> MYNMRRLSLSPTFSMGFHLLVTVSLLFSHVDHVIAETEMEGEGNETGECTGSYYCKKGVILPIWEPQDPSFGDKIARATVYFVAMVYMFLGVSIIADRFMSSIEVITSQEKEITIKKPNGETTKTTVRIWNETVSNLTLMALGSSAPEILLSVIEVCGHNFTAGDLGPSTIVGSAAFNMFIIIALCVYVVPDGETRKIKHLRVFFVTAAWSIFAYTWLYIILSVISPGVVEVWEGLLTFFFFPICVVFAWVADRRLLFYKYVYKRYRAGKQRGMIIEHEGDRPSSKTEIEMDGKVVNSHVENFLDGALVLEVDERDQDDEEARREMARILKELKQKHPDKEIEQLIELANYQVLSQQQKSRAFYRIQATRLMTGAGNILKRHAADQARKAVSMHEVNTEVT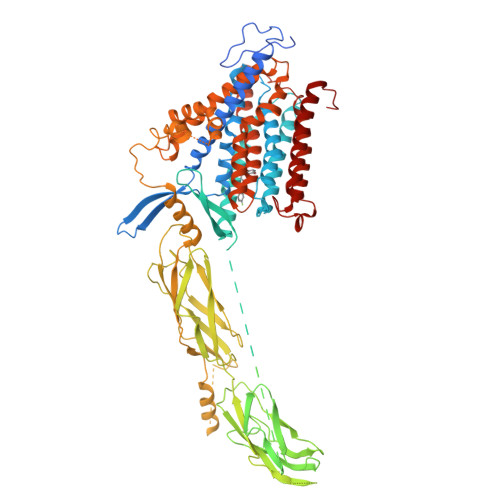ENDPVSKIFFEQGTYQCLENCGTVALTIIRRGGDLTNTVFVDFRTEDGTANAGSDYEFTEGTVVFKPGDTQKEIRVGIIDDDIFEEDENFLVHLSNVKVSSEASEDGILEANHVSTLACLGSPSTATVTIFDDDHAGIFTFEEPVTHVSESIGIMEVKVLRTSGARGNVIVPYKTIEGTARGGGEDFEDTCGELEFQNDEIVKIITIRIFDREEYEKECSFSLVLEEPKWIRRGMKGGFTITDEYDDKQPLTSKEEEERRIAEMGRPILGEHTKLEVIIEESYEFKSTVDKLIKKTNLALVVGTNSWREQFIEAITVSAGEDDDDDECGEEKLPSCFDYVMHFLTVFWKVLFAFVPPTEYWNGWACFIVSILMIGLLTAFIGDLASHFGCTIGLKDSVTAVVFVALGTSVPDTFASKVAATQDQYADASIGNVTGSNAVNVFLGIGVAWSIAAIYHAANGEQFKVSPGTLAFSVTLFTIFAFINVGVLLYRRRPEIGGELGGPRTAKLLTSCLFVLLWLLYIFFSSLEAYCHIKGF> GVSETAPASRRGELAVCDAVSGWVTDRRTAVDLRGREVEVLGEVPAAGGSPLRQYFFETRCKADNAEEGGPGAGGGGCRGVDRRHWVSECKAKQSYVRALTADAQGRVG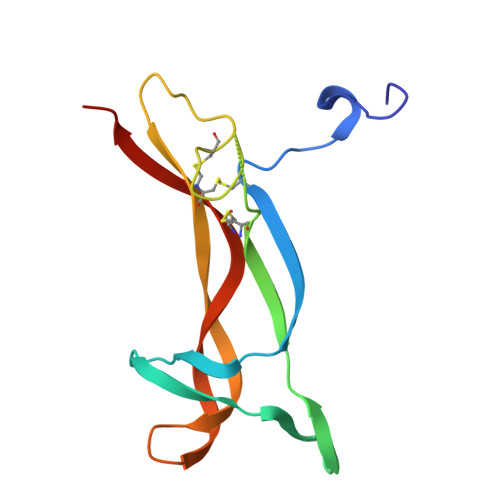WRWIRIDTACVCTLLSRTGRA>GSMDQPAGLQVDYVFRGVEHAVRVMVSGQVLELEVEDRMTADQWRGEFDAGFIEDLTHKTGNFKQFNIFCHMLESALTQSSESVTLDLLTYTDLESLRNRKMGGRPGSLAPRSAQLNSKRYLILIYSVEFDRI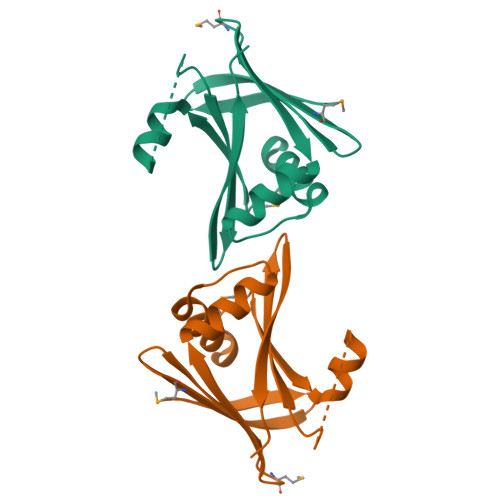HYPLPLPYQGKP[3x]> TIAPI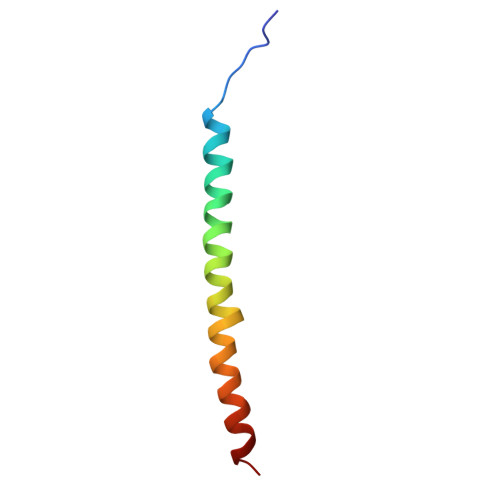TGTIKRRVIMDIVLGFSLGGVMASYWWWGFHMDKINKREKFYAELAE>[2x]MFDMMDAARLEGLHLAQDPATGLKAIIAIHSTRLGPALGGCRYLPYPNDEAAIGDAIRLAQGMSYKAALAGLEQGGGKAVIIRPPHLDNRGA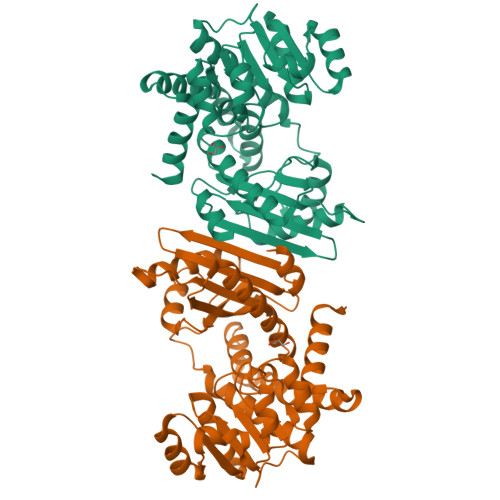LFEAFGRFIESLGGRYITAVDSGTSSADMDCIAQQTRHVTSTTQAGDPSPHTALGVFAGIRASAQARLGSDDLEGLRVAVQGLGHVGYALAEQLAAVGAELLVCDLDPGRVQLAVEQLGAHPLAPEALLSTPCDILAPCGLGGVLTSQSVSQLRCAAVAGAANNQLERPEVADELEARGILYAPDYVINSGGLIYVALKHRGADPHSITAHLARIPARLTEIYAHAQADHQSPARIADRLAERILYGPQHHHHHH2H-IMIDAZOL-4-YLACETIC ACID | C5 H6 N2 O2 | 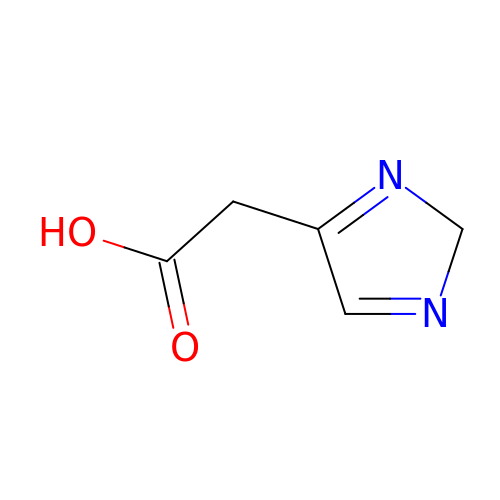RMEAVYUMFHJQAD-UHFFFAOYSA-N> SQSNRELVVDFLSYKLSQKGYSWSQMAAVKQALREAGDEFELRYRRAFSDLTSQLHITPGTAYQSFEQVVNELFRDGVNWGRIVAFFSFGGALCVESVDKEMQVLVSRIAAWMATYLNDHLEPWIQENGGWDTFVELYGN;>SQSNRELVVDFLSYKLSQKGYSWSQMAAVKQALREAGDEFELRYRRAFSDLTSQLHITPGTAYQSFEQVVNELFRDGVNWGRIVAFFSFGGALCVESVDKEMQVL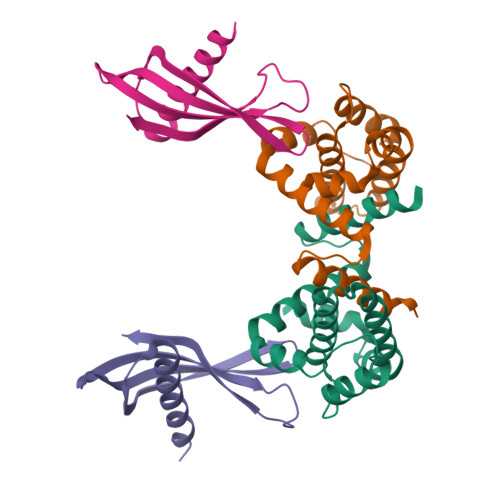VSRIAAWMATYLNDHLEPWIQENGGWDTFVELY[3x];>ENSLEIEELARFAVDEHNKKENALLEFVRVVKAKEQMFSWLDWEETMYYLTLEAKDGGKKKLYEAKVWVKPALLWSPHGNFKELQEFKPV[3x];> SLEIEELARFAVDEHNKKENALLEFVRVVKAKEQMFSWLDWEETMYYLTLEAKDGGKKKLYEAKVWVKPALLWSPHGNFKELQEFKPV> GQ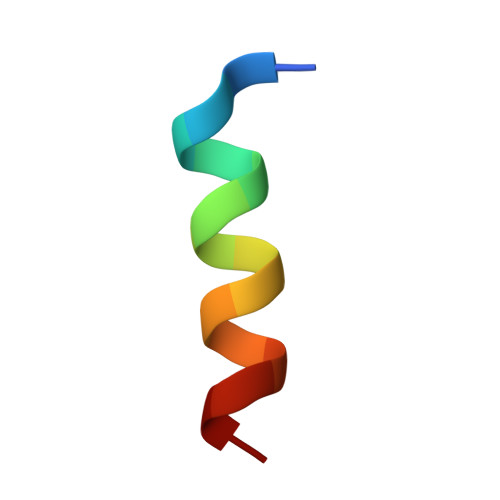VGRQLAIIGDDINR>[2x]GPLGSAQTLQMEIPNFGNSILECLNEQRLQGL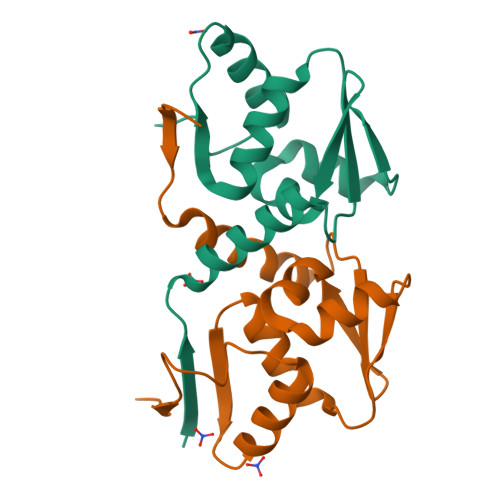YCDVSVVVKGHAFKAHRAVLAASSSYFRDLFNNSRSAVVELPAAVQPQSFQQILSFCYTGRLSMNVGDQDLLMYTAGFLQIQEIMEKGTEFFLKVSS> AEAGITGTWYNQLGSTFIVTAGADGALTGTYESAVGNAESRYVLTGRYDSAPATDGSGTALGWTVAWKNNYRNAHSATTWSGQYVGGAEARINTQ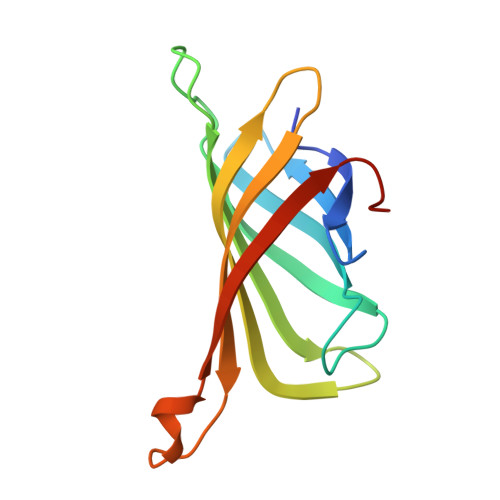WLLTSGTTEANAWKSTLVGHDTFTKVKPSAAS> MTKYYQSLSPTMLGFQEEKFTHLHFYFHDIVTGPKPSMVFVAEPNGKVENALPFGTVVAMDDPLTAGPERDSKLVGKAQGIYTSISQEEMGLMMVMTMAFSDGEFNGSTLSILGRNMIMSETIREMAIVGGTGAFRFVRGYAQAKFFSVDFTTGDATVEYDIFVFHYKGELNSKLEGKP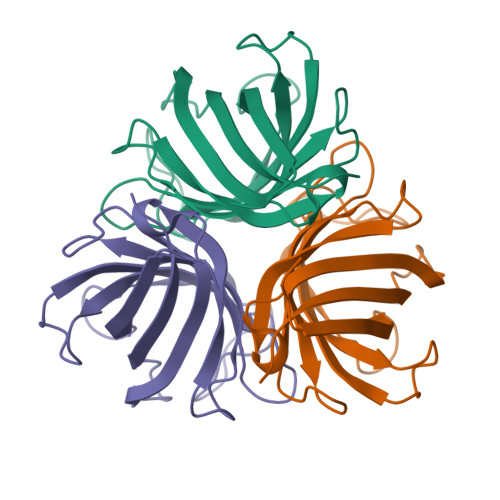IPNPLLGLDSTRTGHHHHHH> MNIFRLTGDLSHLAAIIILLLKIWKSRSCAGISGKSQLLFALVFTTRYLDLFTSFISLYNTSMKLI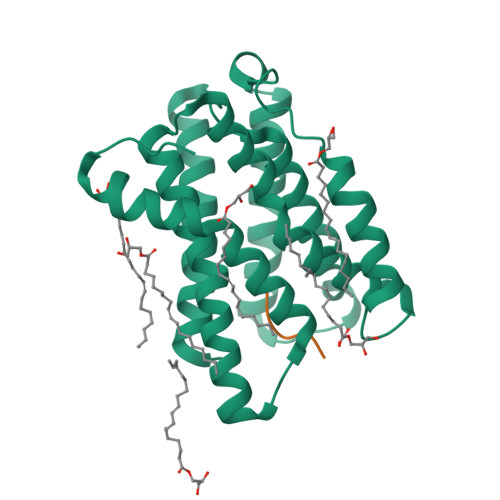YIACSYATVYLIYMKFKATYDGNHDTFRVEFLIVPVGGLSFLVNHDFSPLEILWTFSIYLESVAILPQLFMISKTGEAETITTHYLFFLGLYRALYLVNWIWRYYFEGFFDLIAVVAGVVQTVLYCDFFYLYVTKVLKGKKLSLPA;> EHDEL>MAMLYGKHTHETDETLKPIFGASAERHDLPKYKLAKHALEPREADRLVRDQLLDEGNSRLNLATFCQTYM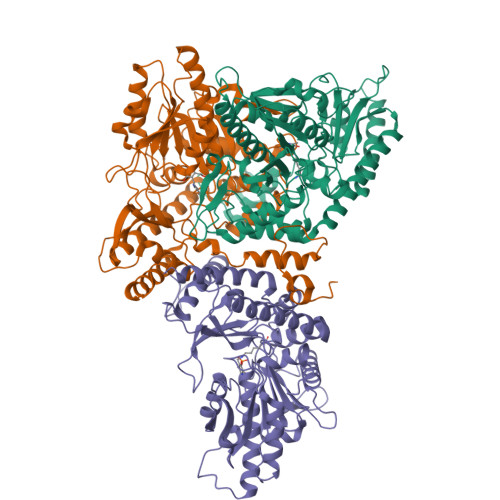EPEAVELMKDTLEKNAIDKSEYPRTAEIENRCVNIIANLWHAPEAESFTGTSTIGSSEACMLAGLAMKFAWRKRAKANGLDLTAHQPNIVISAGYQVCWEKFCVYWDIDMHVVPMDDDHMSLNVDHVLDYVDDYTIGIVGIMGITYTGQYDDLARLDAVVERYNRTTKFPVYIHVDAASGGFYTPFIEPELKWDFRLNNVISINASGHKYGLVYPGVGWVIWRDQQYLPKELVFKVSYLGGELPTMAINFSHSASQLIGQYYNFIRFGFDGYREIQEKTHDVARYLAKSLTKLGGFSLINDGHELPLICYELTADSDREWTLYDLSDRLLMKGWQVPTYPLPKNMTDRVIQRIVVRADFGMSMAHDFIDDLTQAIHDLDQAHIVFHSDPQPKKYGFTH[3x]> GSSPQHLLVGGSGWNKIAIINKDTKEIVWEYPLEKGWECNSVAATKAGEILFSYSKGAKMITRDGRELWNIAAPAGCEMQTARILPDGNALVAWCGHPSTILEVNMKGEVLSKTEFETGIERPHAQFRQINKNKKGNYLVPLFATSEVREIAPNGQLLNSVKLSGTPFSSAFLDNGDCL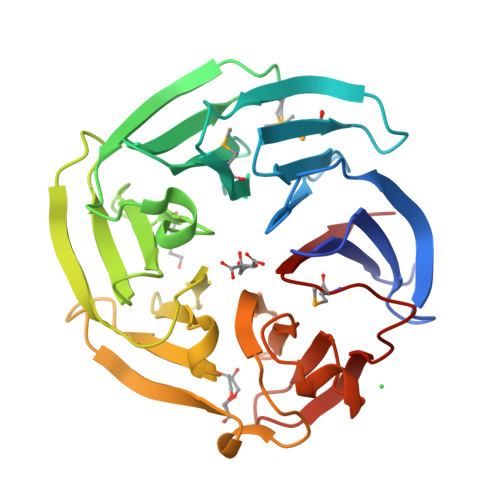VACGDAHCFVQLNLESNRIVRRVNANDIEGVQLFFVAQLFPLQNGGLYICNWQGHDREAGKGKHPQLVEIDSEGKVVWQLNDKVKFGMISTICPIRE>MTTNTIMEQEARTAPQKIAEQLLANDAITESLGSVLREFKPKFVMIVGRGSSDHAGVFAKYLFEIEASIPTFAAAPSVASVYGKTLKLAGGLVIVISQSGRSPDILAQARMAKNAGAFCVALVNDETAPIKDIVDVVIPLRAGEEKAVAATKSYLATLSALLQVAAKWTQNESLVEAVNSLPQALQAAVDAEPQLRAGSLTDVKNLVVLGRGFGYAVSKEIALKLKEVCAIHAEAFSSAEFLHGPVTLVEKKLSILDVCIRDESYGSHVEQIANVKQRGANLIHLHQTSADIHPRIAPLALLQRFYIDVAAVAIA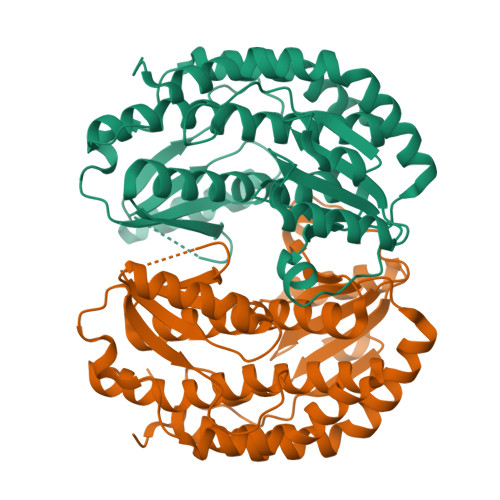LGINPDKPAGLKKVTQTL[2x]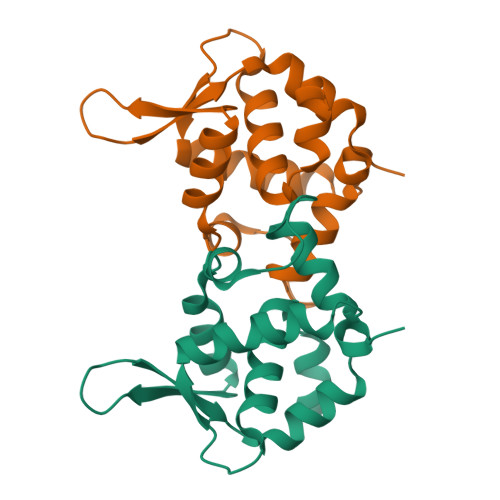> GPSEAINGFKDETISKKIIGMSLLMRTFLYTLAQETEGTNRHTLALETVLIKMVKMLRDNPGYKASKEIKKVICGAWEPAITIEKLKQFSWISVVNDLVGEKLVVVVLEEPSASIMVELKLPLEINYAFSMDEEFKNMDCI>MNLIPTVIETTNRGERAYDIYSRLLKDRIIMLGSQIDDNVANSIVSQLLFLQAQDSEKDIYLYINSPGGSVTAGFAIYDTIQHIKPDVQTICIGMAASMGSFLLAAGAKGKRFALPNAEVMIHQPLGGAQGQATEIEIAANHILKTREKLNRILSERTGQSIEKIQQDTDRDNFLTAAEAKEYGLIDEVMEPEKHHH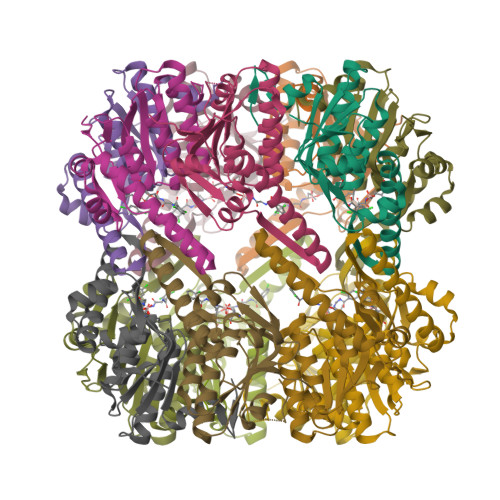HHH[14x]2-phenylethyl (2E)-3-(3,4-dihydroxyphenyl)prop-2-enoate 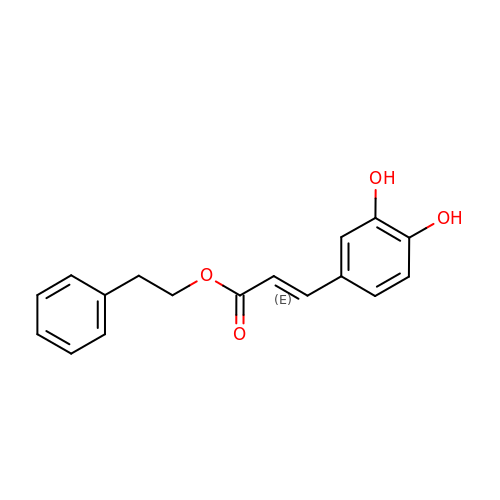| C17 H16 O4 | SWUARLUWKZWEBQ-VQHVLOKHSA-N> AAGVAAWLPFARAAAIGWMPVASGPMPAPPRQERKRTQDALIVLNVSGTRFQTWQDTLERYPDTLLGSSERDFFYHPETQQYFFDRDPDIFRHILNFYRTGKLHYPRHECISAYDEELAFFGLIPEIIGDCCYEEYKDRRRENAERLQDDADTDTAGESALPTMTARQRVWRAFENPHTSTMALVFYYVTGFFIAVSVIANVVETVPCGSSPGHIKELPCGERYAVAFFCLDTACVMIFTVEYLLRLAAAPSRYRFVRSVMSIIDVVAILPYYIGLVMTDNEDVSGAFVTLRVFRVFRIFKFSRHSQGLRILGYTLKSCASELGFLLFSLTMAIIIFATVMFYAEKGSSASKFTSIPAAFWYT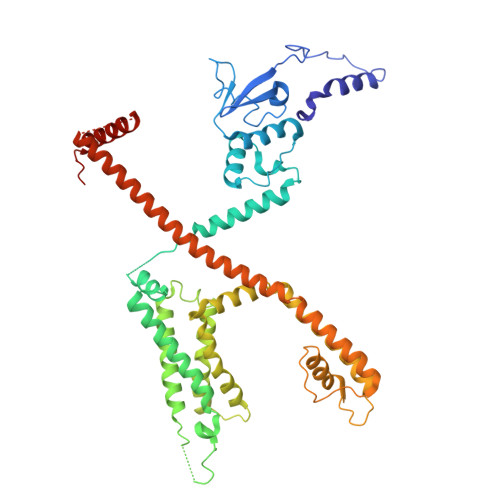IVTMTTLGYGDMVPKTIAGKIFGSICSLSGVLVIALPVPVIVSNFSRIYHQNQRADKRRAQKKARLARIRAAKSGSANAYMQSKRSGLLSNQLQSSEDEQAFVSKSGSSFETQHHHLLHCLEKTTNHEFVD> 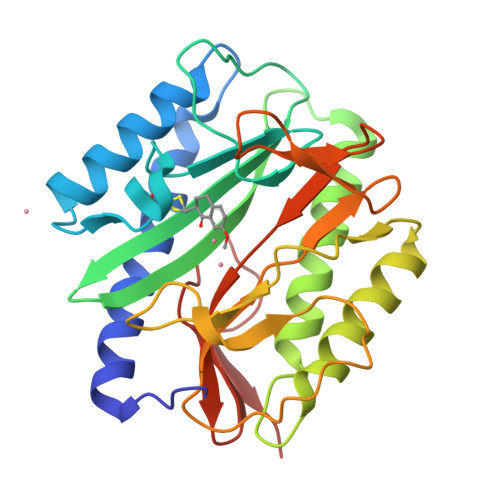MAISIKTPEDIEKMRVAGRLAAEVLEMIEPYVKPGVSTGELDRICNDYIVNEQHAVSACLGYHGYPKSVCISINEVVCHGIPDDAKLLKDGDIVNIDVTVIKDGFHGDTSKMFIVGKPTIMGERLCRITQESLYLALRMVKPGINLREIGAAIQKFVEAEGFSVVREYCGHGIGQGFHEEPQVLHYDSRETNVVLKPGMTFTIEPMVNAGKKEIRTMKDGWTVKTKDRSLSAQYEHTIVVTDNGCEILTLRKDDTIPAIISHDE>[2x]KHLINDDFNETALLLAFKQNSVKSDPNNVLGNWKYESGRGSCSWRGVSCSDDGRIVGLDLRNSGLTGTLNLVNLTALPNLQNLYLQGNYFSSGGDSSGSDCY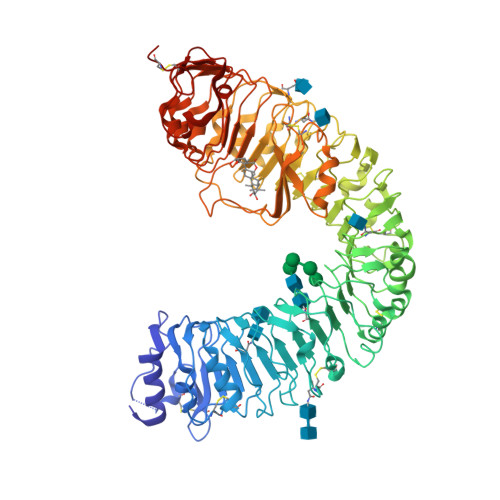LQVLDLSSNSISDYSMVDYVFSKCSNLVSVNISNNKLVGKLGFAPSSLQSLTTVDLSYNILSDKIPESFISDFPASLKYLDLTHNNLSGDFSDLSFGICGNLTFFSLSQNNLSGDKFPITLPNCKFLETLNISRNNLAGKIPNGEYWGSFQNLKQLSLAHNRLSGEIPPELSLLCKTLVILDLSGNTFSGELPSQFTACVWLQNLNLGNNYLSGDFLNTVVSKITGITYLYVAYNNISGSVPISLTNCSNLRVLDLSSNGFTGNVPSGFCSLQSSPVLEKILIANNYLSGTVPMELGKCKSLKTIDLSFNELTGPIPKEIWMLPNLSDLVMWANNLTGTIPEGVCVKGGNLETLILNNNLLTGSIPESISRCTNMIWISLSSNRLTGKIPSGIGNLSKLAILQLGNNSLSGNVPRQLGNCKSLIWLDLNSNNLTGDLPGELASQAGLVMPGSVSGKQFAFVRNEGGTDCRGAGGLVEFEGIRAERLERLPMVHSCPATRIYSGMTMYTFSANGSMIYFDISYNAVSGFIPPGYGNMGYLQVLNLGHNRITGTIPDSFGGLKAIGVLDLSHNNLQGYLPGSLGSLSFLSDLDVSNNNLTGPIPFGGQLTTFPVSRYANNSGLCGVPLRPCGSAHHHHHH> DQGRGRRRP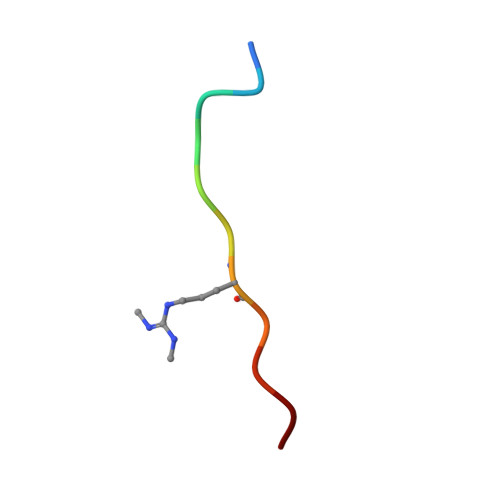LN>[3x]GAMDYSLVKALQTAQQNFVISDPSIPDNPIVYASQGFLTLTGYALSEVLGRNCRFLQGPETDPKAVEKVRKGLERGEDTTVVLLNYRKDGSTFWNQLFIAALRDGEGNVVNYLGVQCKVSEDYAKAFLKNEENE;> GAMDYSLVKALQTAQQNFVISDPSIPDNPIVYASQGFLTLTGYALSEVLGRNCRFLQGPETDPKAVEKVRKGLERGEDTTVVLLNYRKDG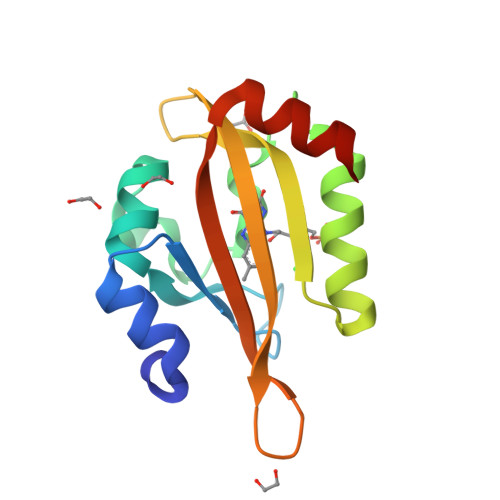STFWNQLFIAALRDGEGNVVNYLGVQCKVSEDYAKAFLKNEEKE9-beta-D-ribofuranosyl-6-(thiophen-3-yl)-9H-purine 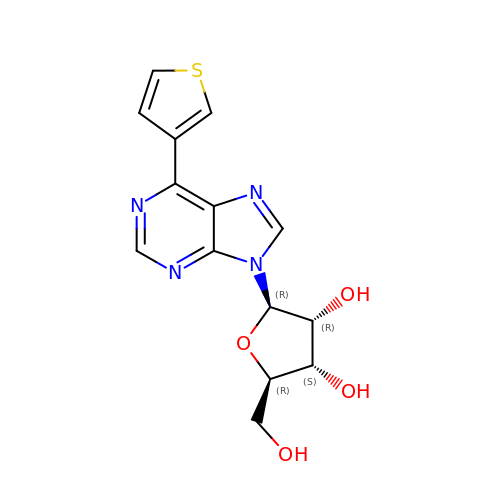| C14 H14 N4 O4 S | UXKNTUXJYSDVTH-LHNIVKCTSA-N> MNSPISPIETVPVKLKPGMDGPKVKQWPLTEEKIKALVEICTEMEKEGKISKIGPENPYNTPVFAIKKKDSTKWRKLVDFRELNKRTQDFWEVQLGIPHPAGLKKNKSVTVLDVGDAYFSVPLDEDFRKYTAFTIPSINNETPGIRYQYNVLPQGWKGSPAIFQSSMTKILEPFRKQNPDIVIYQYMDDLYVGSDLEIGQHRTKIEELRQHLLRWGLTTPDKKHQKEPPFLWMGYELHPDKWTVQPIVLPEKDSWTVNDIQKLVGKLNWASQIYPGIKVRQLCKLLRGTKALTEVIPLTEEAELELAENREILKEPVHGVYYDPSKDLIAEIQKQGQGQWTYQIYQEPFKNLKTGKYARMRG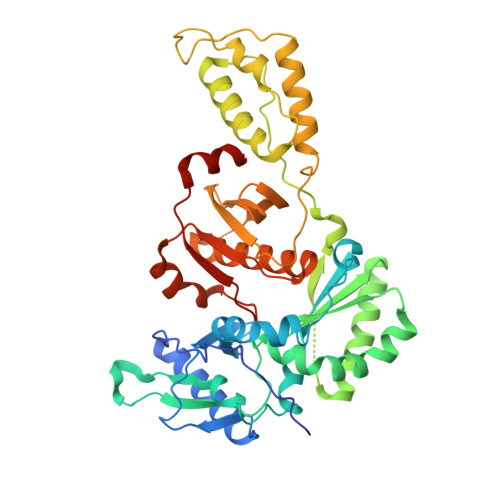AHTNDVKQLTEAVQKITTESIVIWGKTPKFKLPIQKETWETWWTEYWQATWIPEWEFVNTPPLVKLWYQLEKEPIVGAETF>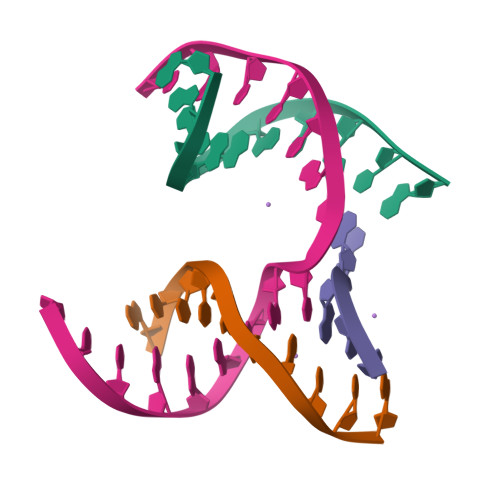 GAGCAGACGTG;> ACTGCACTCA;> CAAGT;> TCTGAGTGCCGTCTGC> MGATGDAEQPRGPSGAERGGLELGDAGAAGQLVLTNPWNI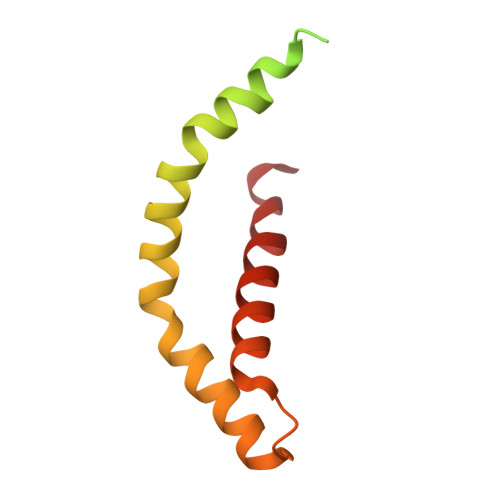MIKHRQVQRRGRRSQMTTSFTDPAISMDLLRAVLQPSINEEIQTVFNKYMKFFQKAALNVRDNVGEEVDAEQLIQEACRSCLEQAKLLFS> MTSENPDVLLSRVINVVRAAS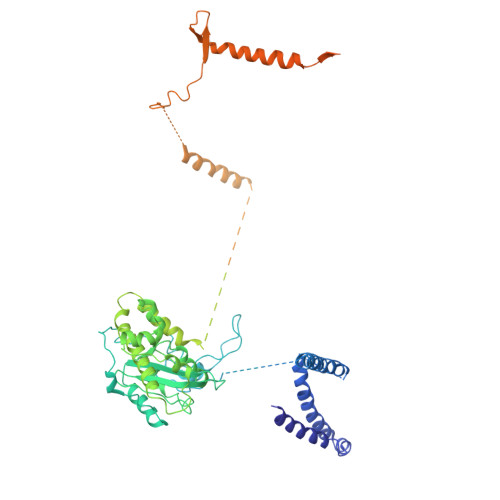SLASQDVDFYKNLDRGFSKDLKSKADKLADMANEIILSIDEHHESFELKEEDISDLWNNFGNIMDNLLEMSDHSLDKLNCAINSKSRGSDLQYLGEFSGKNFSPTKRVEKPQLKFKSPIDNSESHPFIPLLKEKPNALKPLSESLRLVDDDENNPSHYPHPYEYEIDHQEYSPEILQIREEIPSKSWDDSVPIWVDTSTELESMLEDLKNTKEIAVDLEHHDYRSYYGIVCLMQISTRERDYLVDTLKLRENLHILNEVFTNPSIVKVFHGAFMNIIWLQRDLGLYVVGLFDTYHASKAIGLPRHSLAYLLENFANFKTSKKYQLADWRIRPLSKPMTAYARADTHFLLNIYDQLRNKLIESNKLAGVLYESRNVAKRRFEYSKYRPLTPSSEVYSPIEKESPWKILMYQYNIPPEREVLVRELYQWRDLIARRDDESPRFVMPNQLLAALVAYTPTDVIGVVSLTNGVTEHVRQNAKLLANLIRDALRNIKNTNEEATPIPSSETKADGILLETISVPQIRDVMERFSVLCNSNISKSRAKPVTNSSILLGKILPREEHDIAYSKDGLPNKVKTEDIRIRAQNFKSALANLEDIIFEIEKPLVVPVKLEEIKTVDPASAPNHSPEIDNLDDLVVLKKKNIQKKQPAKEKGVTEKDAVDYSKIPNILSNKPGQNNRQQKKRRFDPSSSDSNGPRAAKKRRPAAKGKNLSFKR>GAMASTHHTMKIRSTKFSILNSDHPRIEVKKVFSLSPDVQVTIPYRRFKGKAKVYFQNDQIQGYFSCTDRQIDEIKISAPKNAPLLEPLLDICYYGSFIEPGFEQTFGFYPAGKREFVDSFFMHHSKDHKAFLIHMGLDKDLSLPLSPELNWKEPALSKVCRVTELDS[2x]

The three largest gene segments of the Thogotoviruses, THOV, DHOV and JOSV are homologous to those of IAV and code for the heterotrimeric polymerase. In this paper we present the atomic structures of the putative PB2 cap binding and 627 domains of THOV and the putative PA N-terminal endonuclease domains of THOV and DHOV. Despite very low sequence homologies, all domains have similar folds to those of the corresponding IAV polymerase domains. However, the critical active site residues in the putative cap binding and endonuclease domains are not conserved in THOV and DHOV and, contrary to the case of IAV polymerase, neither domain shows the expected in vitro biochemical activity.

A construct comprising residues 323–486 could be expressed, crystallised in two different forms, and its structure determined at 1.8 Å resolution. Firstly, the so called ‘348-loop’ formed by the β3–β4 hairpin is longer in THOV and its extremity orientates away from the body of the domain towards the solvent, whereas in IAV the tip packs against bends the body of the molecule. This is apparently not an artefact of crystal packing as a very similar conformation of this beta hairpin is observed in the second crystal form. Finally, in all three crystallographically independent examples of the THOV domain, the equivalent position of the m7G itself is occupied by the side-chain of Arg344, with its guanidinium group stacking with the side-chain and making two hydrogen bonds to the main-chain carbonyl oxygen of Tyr413. Furthermore, given the high resolution, well-ordered structure of the THOV domain, which is the same for all three crystallographically independent copies observed, it is extremely unlikely that the putative active site region could be repacked through induced fit to allow m7G binding. Thus the significantly different nature and arrangement of the residues within the putative active site of THOV would appear to preclude any possible binding of m7G in a similar manner to that observed in IAV. The THOV domain is not retained by m7G Sepharose under conditions where IAV cap-binding domain is and, similarly, no binding of m7GTP could be detected by isothermal calorimetry experiments under conditions where IAV cap-binding domain shows clear binding with a Kd of 2.7 µM.>[2x]UUGCGU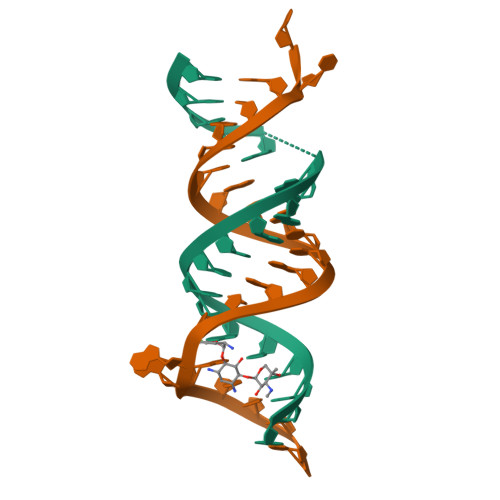CACGCCGGCGAAGUCGC> NNPYLFRSNKFLTLFKNQHGSLRLLQRFNEDTEKLENLRDYRVLEYCSKPNTLLLPHHSDSDLLVLVLEGQAILVLVNPDGRDTYKLDQGDAIKIQAGTPFYLINPDNNQNLRILKFA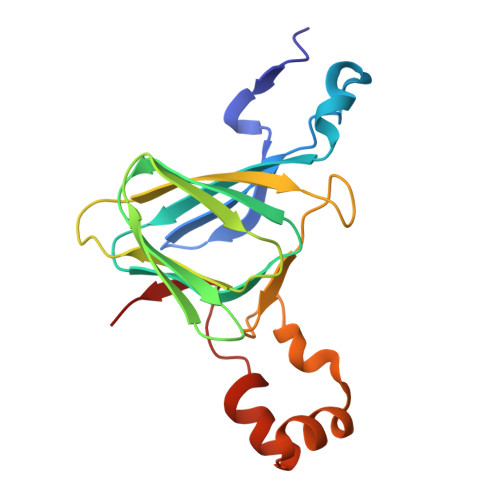ITFRRPGTVEDFFLSSTKRLPSYLSAFSKNFLEASYDSPYDEIEQTLLQEEQEGVIVKMP>[5x]VSPPPPIADEPLTVNTGIYLIECYSLDDKAETFKVNAFLSLSWKDRRLAFDPVRSGVRVKTYEPEAIWIPEIRFVNVENARDADVVDISVSPDGTVQYLERFSARVLSPLDFRRYPFDSQTLHIYLIVRSVDTRNIVLAVDLEKVGKNDDVFLT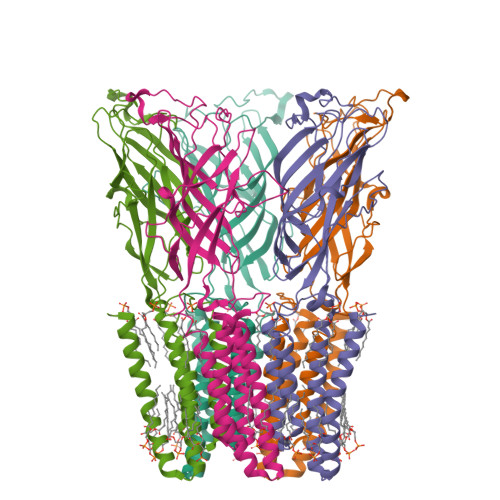GWDIESFTAVVKPANFALEDRLESKLDYQLRISRQYFSYIPNIILPMLFILFISWTAFWSTSYEANVTLVVSTLIAHIAFNILVETNLPKTPYMTYTGAIIFMIYLFYFVAVIEVTVQHYLKVESQPARAASITRASRIAFPVVFLLANIILAFLFFGF>[6x]SNAMSTIARRGFHYMQRLNSANVSPALLEKAQNRVIDAALTFIRERAKFKGELMRSLGGVAATSSLLGVPLGHHSSFHEGSAFAPPRIREAIWCDSTNSTTEEGKNLRDPRVITNVGDVPIEEIRDCGVDDKRLANVISESVKLVMDEDPLRPLVLGGDHSISFPVVRAVSEKLGGAVDILHFDAHPDLYHDFEGNYYSHASPFARIMEGGYARRLVQVGIRSITNDVREQVKKYGVETHEMRTLSRDRPILENLKLGEGVKGVYVSIDVDSLDPSIAPGVSHHEPGGLLFRDILNILQNLQGDIVGGDVVEYNPQRDTYDGITALVAAKLVRELAAKMSK

In this route, ornithine is obtained from arginine by the action of arginase (arginine amidinohydrolase, ARGAH). Similarly to other eukaryotic (Di Costanzo et al., 2010) and prokaryotic (Bewley et al., 1999) orthologues, plant ARGAHs, are binuclear manganese metalloenzymes. Together with agmatinase, formiminoglutamase, and proclavaminate aminohydrolase, ARGAHs are grouped with the Ureohydrolase Superfamily.

In this work, ARGAHs from two model plant species, A. thaliana (AtARGAH1) and Medicago truncatula (MtARGAH), are structurally characterized by X-ray crystallography and small-angle X-ray scattering (SAXS).> MSITL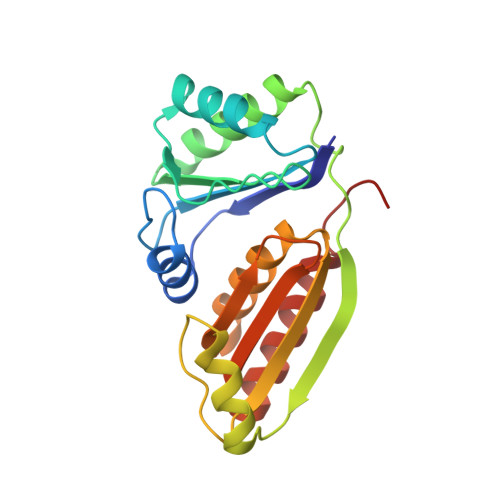RTYIFLDALQPQLATFIGKTARGFLPVPGQASLWVEIAPGIAINRVTDAALKATKVQPAVQVVERAYGLLEVHHFDQGEVLAAGSTILDKLEVREEGRLKPQVMTHQIIRAVEAYQTQIINRNSQGMMILPGESLFILETQPAGYAVLAANEAEKAANVHLVNVTPYGAFGRLYLAGSEAEIDAAAEAAEAAIRSVSGVA> XVTVDQDLLDAAGILPFE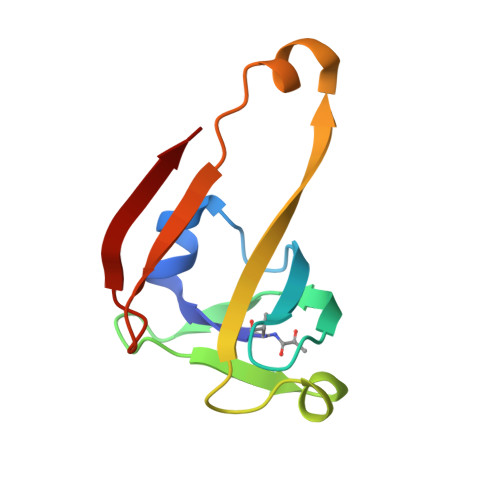QVDIYDITNGARLTTYALPGERGSGVIGINGAAAHLVKPGDLVILVAYGVFDEEEARNLKPTVVLVDERNRILEVRKG>GSYGSSSQSSSYGQPQSGS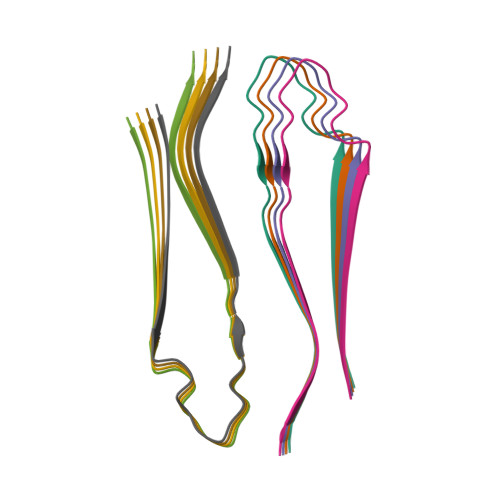YSQQPSYGGQQQSYGQQQSYNPPQGYGQQNQYNSSSGGGGGGGGGGNYGQDQSSMSSGGGSGGGYGNQDQSGGGGSGGYGQGDRG[8x]>[4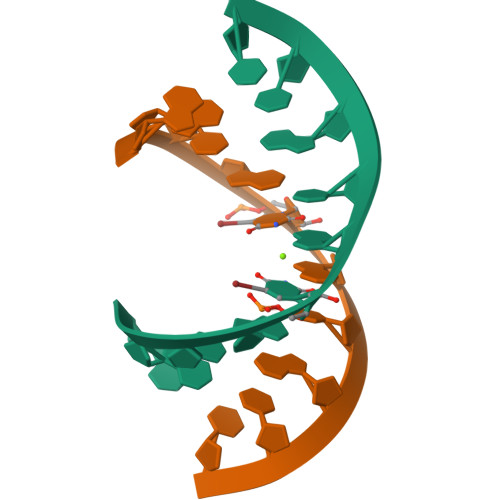x]GGCGUGCGCU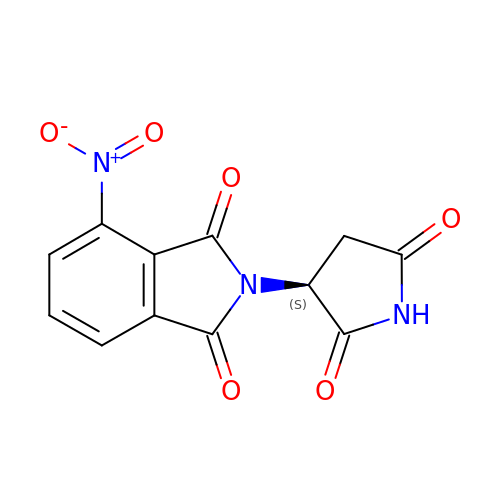2-[(3~{S})-2,5-bis(oxidanylidene)pyrrolidin-3-yl]-4-nitro-isoindole-1,3-dione | C12 H7 N3 O6 | NSOHSQDNWATGPD-ZETCQYMHSA-N Asparaginases (EC 3.5.1.1), which split L-asparagine to L-aspartate and ammonia, are grouped into three unrelated structural classes: Class 1 (bacterial-type), Class 2 (plant-type), and Class 3 (Rhizobium etli-type). ReAV is a homodimer with an α/β protomeric fold, formed by two tightly packed domains. The active site of the enzyme is located in a cleft on the protomer surface and marked by a zinc ion with an unusual coordination sphere created by Cys135, Lys138, Cys189, and a water molecule. The conspicuous catalytic center of the enzyme comprises two Ser-Lys tandems (Ser48-Lys51 and Ser80-Lys263), centered around the curiously hydrated Ser48 residue and located in the close vicinity of the metal binding site.

The substitution of Lys138 with alanine caused significant structural rearrangements in the active site region. In the presence of the Lys138 mutation, the coordination site fell apart and is no longer accentuated by the metal cation. The absence of Lys138 affected the position and conformational states of Ser48 and Lys51 from the Ser48-Lys51 tandem, disrupting the H-bond network in the active site area, as well as the conformation of the cysteine residues from the zinc coordination sphere. In the four protein chains, the metal site was filled with a water molecule (w1) bound by the Sγ atoms of Cys135 and Cys189, and additionally, in protein chain C, alternative conformers of Cys135 and Cys189 form a direct Cys135-Cys189 disulfide bridge. The Ser48 side chain has a slightly different position depending on the protein chain, without the characteristic pattern of three closely-spaced water molecules. The absence of Lys138 evidently impaired the mutant’s ability to bind the Zn2+ cation. Interestingly, the collapse of the metal binding site did not abolish the L-asparaginase activity of the mutant protein completely, as 1.5% of the activity (in terms of kcat/KM) was still observed (vide supra). Moreover, as shown by ITC affinity studies, the K138A mutant is still able to bind the zinc ion, albeit with lower affinity (∼26 μM) than the WT protein (∼3 μM). The low zinc binding affinity explains the absence of the zinc ion in the crystal structure. 10 μM Zn2+ greatly improves the KM of ReAV K138A from 2.2 to 0.5 mM, making this mutant an excellent candidate for substrate co-crystallization experiments, and indeed for further optimization toward antileukemic properties.

>[4x]GIDPFTMTPSEDFVVTDRGGIVENSHRVHAAVVDAKGRLLYALGNPTRMTLARSAAKPAQALAILETEGVAGYGFDDADIALMCASHSSEDRHIARTRAMLSKIKAEEADLRCGGHPSLSEMVNRSWIKQDFIPTAVCSNCSGAHVGMLAGARAIGAGTDGYHLPDHPMQGRVKRTVAELCDLDAGDVEWGTDGCNLPTPAFPLDRLGRIYAKLASAADGSDAGEGQSTRCAALAHIFRAMARHPEMVAGEGRYCTMLMRAFDGALVGKLGADASYAIGVRASDATRQLGTDGALGISVKIEDGNLEMLYAVVTELLERLGIGSPDVRSQLASFHHPQRVNTMGVTTGGVSFPFKLRGSKSNVDDPRLAAVAR>[2x]MGSDKIHHHHHHMDTRKNVSGAERKIWSLIRDCSGKLEGVTETSVLEVLLIVSRVLGIRKEDLFLKDLGVSPTEEKRILELVEKRASGYPLHYILGEKEFMGLSFLVEEGVFVPRPETEELVELALELIRKYGIK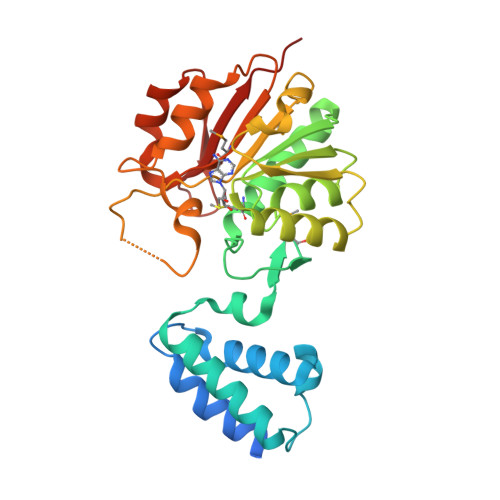TVADIGTGSGAIGVSVAKFSDAIVFATDVSSKAVEIARKNAERHGVSDRFFVRKGEFLEPFKEKFASIEMILSNPPYVKSSAHLPKDVLFEPPEALFGGEDGLDFYREFFGRYDTSGKIVLMEIGEDQVEELKKIVSDTVFLKDSAGKYRFLLLNRRSS> VTAFLGERVTLTSYWRRVSLGPEIEVSWFKLGPGEEQVLIGRMHHDVIFIEWPFRG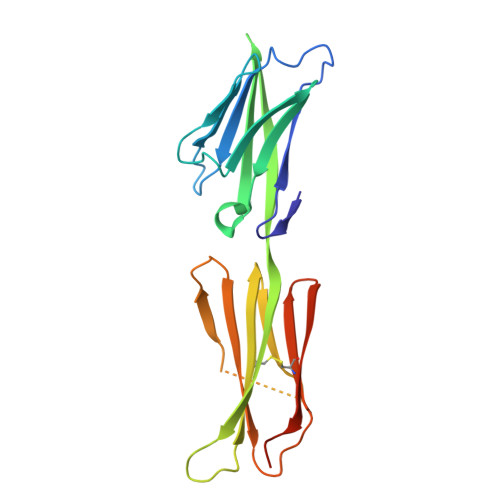FFDIHRSANTFFLVVTAANISHDGNYLCRMKLGETEVTKQEHLSVVKPLTLSVHSERSQFPDFSVLTVTCTVNAFPHPHVQWLMPEGVEPAPSAANGGVMKEKDGSLSVAVDLSLPKPWHLPVTCVGKNDKEEAHGVYVSGYLSQKHHHHHH> PHVICEPCIGVKD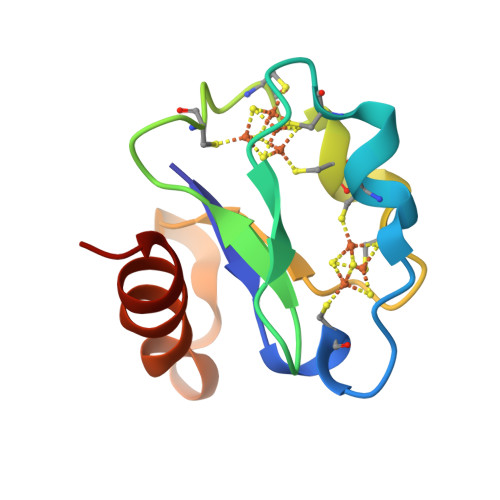QSCVEVCPVECIYDGGDQFYIHPEECIDCGACVPACPVNAIYPEEDVPEQWKSYIEKNRKLAGLE> MAIYTVKALITDPIDEILIKTLREKGIQVDYMPEISKEELLNIIGNYDIIVVRSRTKVTKDVIEKGKKLKIIARAGIGLDNIDTEEAEKRNIKVVYAPGASTDSAVELTIGLMIAAARKMYTSMALAKSGIFKKIEGLELAGKTIGIVGFGRIGTKVGIIANAMGMKVLAYDILDIREKAEKINAKAVSLEELLKNSDVISLHVTVSKDAKPIIDYPQFELMKDNVIIVNTSRAVAVNGKALLDYIKKGKVYAYATDVFWNEP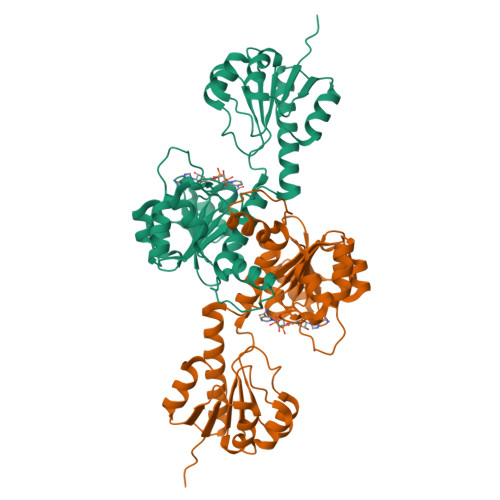PKEEWELELLKHERVIVTTHIGAQTKEAQKRVAEMTTQNLLNAMKELGMI> GSEVRSDRDKFVIFLDVKHFSPEDLTVKVQEDFVEIHGKHNERQDD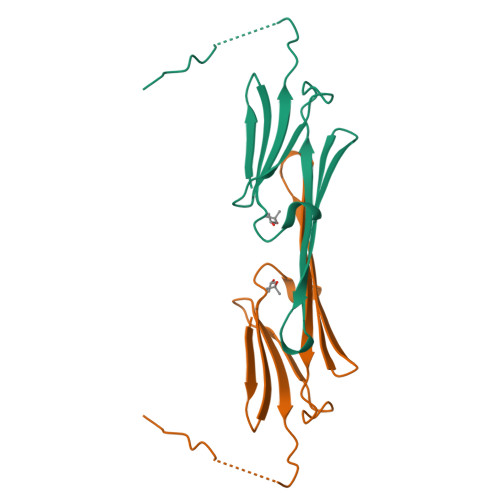HGYISREFHRRYRLPSNVDQSALSCSLSADGMLTFSGPKIPSGVDAGHSERAIPVSR> SMSDTLTIGLQKKPGKGLGLSIVGKRNDTGVFVSDIV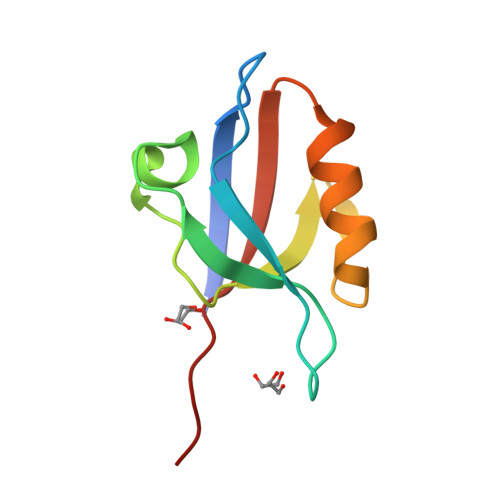KGGIADADGRLMQGDQILMVNGEDVRNATQEAVAALLKCSLGTVTLEVGRISTYV> AGSEQLKCCSGILKEMFAK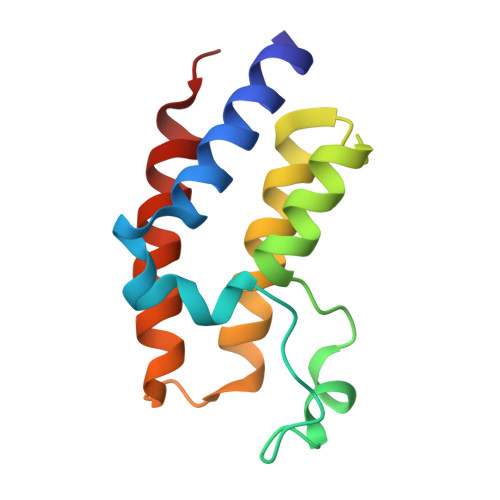KHAAYAWPFYKPVDVEALGLHDYCDIIKHPMDMSTIKSKLEAREYRDAQEFGADVRLMFSNCYKYNPPDHEVVAMARKLQDVFEMRFAKMPD> MEDVEIKPRGYQLRLVDHLTKSNGIVYLPTGSGKTFVAILVLKRFSQDFDKPIESGGKRALFMCNTVELARQQAMAVRRCTNFKVGFYVGEQGVDDWTRGMWSDEIKKNQVLVGTAQVFLDMVTQTYVALSSLSVVIIDECHHGTGHHPFREFMRLFTIANQTKLPRVVGLTGVLIKGNEITNVATKLKELEITYRGNIITVSDTKEMENVMLYATKPTEVMVSFPHQEQVLTVTRLISAEIEKFYVSLDLMNIGVQPIRRSKSLQCLRDPSKKSFVKQLFNDFLYQMKEYGIYAASIAIISLIVEFDIKRRQAETLSVKLMHRTALTLCEKIRHLLVQKLQDMTYDDDDDNVNTEEVIMNFSTPKVQRFLMSLKVSFADKDPKDICCLVFVERRYTCKCIYGLLLNYIQSTPELRNVLTPQFMVGRNNISPDFESVLERKWQKSAIQQFRDGNANLMICSSVLEEGIDVQACNHVFILDPVKTFNMYVQSKGRARTTEAKFVLFTADKEREKTIQQIYQYRKAHNDIAEYLKDRVLEKTEPELYEIKGHFQDDIDPFTNENGAVLLPNNALAILHRYCQTIPTDAFGFVIPWFHVLQEDERDRIFGVSAKGKHVISINMPVNCMLRDTIYSDPMDNVKTAKISAAFKACKVLYSLGELNERFVPKTLKERVASIADVHFEHWNKYGDSVTATVNKADKSKDRTYKTECPLEFYDALPRVGEICYAYEIFLEPQFESCEYTEHMYLNLQTPRNYAILLRNKLPRLAEMPLFSNQGKLHVRVANAPLEVIIQNSEQLELLHQFHGMVFRDILKIWHPFFVLDRRSKENSYLVVPLILGAGEQKCFDWELMTNFRRLPQSHGSNVQQREQQPAPRPEDFEGKIVTQWYANYDKPMLVTKVHRELTPLSYMEKNQQDKTYYEFTMSKYGNRIGDVVHKDKFMIEVRDLTEQLTFYVHNRGKFNAKSKAKMKVILIPELCFNFNFPGDLWLKLIFLPSILNRMYFLLHAEALRKRFNTYLNLHLLPFNGTDYMPRPLEIDYSLKRNVDPLGNVIPTEDIEEPKSLLEPMPTKSIEASVANLEITEFENPWQKYMEPVDLSRNLLSTYPVELDYYYHFSVGNVCEMNEMDFEDKEYWAKNQFHMPTGNIYGNRTPAKTNANVPALMPSKPTVRGKVKPLLILQKTVSKEHITPAEQGEFLAAITASSAADVFDMERLEILGDSFLKLSATLYLASKYSDWNEGTLTEVKSKLVSNRNLLFCLIDADIPKTLNTIQFTPRYTWLPPGISLPHNVLALWRENPEFAKIIGPHNLRDLALGDEESLVKGNCSDINYNRFVEGCRANGQSFYAGADFSSEVNFCVGLVTIPNKVIADTLEALLGVIVKNYGLQHAFKMLEYFKICRADIDKPLTQLLNLELGGKKMRANVNTTEIDGFLINHYYLEKNLGYTFKDRRYLLQALTHPSYPTNRITGSYQELEFIGDAILDFLISAYIFENNTKMNPGALTDLRSALVNNTTLACICVRHRLHFFILAENAKLSEIISKFVNFQESQGHRVTNYVRILLEEADVQPTPLDLDDELDMTELPHANKCISQEAEKGVPPKGEFNMSTNVDVPKALGDVLEALIAAVYLDCRDLQRTWEVIFNLFEPELQEFTRKVPINHIRQLVEHKHAKPVFSSPIVEGETVMVSCQFTCMEKTIKVYGFGSNKDQAKLSAAKHALQQLSKCDA;> MDQENFHGSSLPQQLQNLHIQPQQASPNPVQTGFAPRRHYNNLVGLGNGNAVSGSPVKGAPLGQRHVKLKKEKISAQVAQLSQPGQLQLSDVGDPALAGGSGLQGGVGLMGVILPSDEALKFVSETDANGLAMKTPVSILQELLSRRGITPGYELVQIEGAIHEPTFRFRVSFKDKDTPFTAMGAGRSKKEAKHAAARALIDKLIGAQLPESPSSSAGPSVTGLTVAGSGGDGNANATGGGDASDKTVGNPIGWLQEMCMQRRWPPPSYETETEVGLPHERLFTIACSILNYREMGKGKSKKIAKRLAAHRMWMRLQETPIDSGKISDSICGELEGEVSIIQDIDRYEQVSKDFEFIKI

In Drosophila, an RNase III enzyme Dicer-2 (Dcr-2), aided by its cofactor Loquacious-PD (Loqs-PD), has an important role in generating 21 bp siRNA duplexes from long double-stranded RNAs (dsRNAs). ATP hydrolysis by the helicase domain of Dcr-2 is critical to the successful processing of a long dsRNA into consecutive siRNA duplexes. Here six cryo-electron microscopy (cryo-EM) structures of Drosophila Dcr-2–Loqs-PD in apo and in complex with dsRNA substrate in the absence or in the presence of ATP were captured, illuminating the continuous conformational changes of Dcr-2–Loqs-PD after binding to dsRNA and translocating until forming the active dicing state and cleaving the dsRNA substrate into an siRNA duplex in the post-dicing state. Loqs-PD is a cofactor protein that comprises two dsRBDs that are responsible for recruiting siRNA precursor substrates for Dcr-2.

To investigate the dynamic dicing process of Dcr-2, we mixed WT Dcr-2–Loqs-PD with a 50 bp dsRNA substrate, then added ATP and Mg2+ just before generating the cryo-EM samples. From such an enzymatically active sample, we were able to capture a complex structure in the post-dicing state at a relatively lower resolution (4.6 Å). In this structure, a clear breakage of the dsRNA after the dicing near to the catalytic centre was observed and exactly 21 bp away from the PAZ-domain-binding terminus. The cleavage of dsRNA disrupts the binding site for the C-terminal dsRBD in the active dicing state, and probably results in the dsRBD becoming more flexible and losing its density in the averaged EM map of the post-dicing state, which may be also favourable to the release of cleaved siRNA products. Compared with the structure in the active dicing state, the cap–core module with siRNA in the post-dicing state rotated about 20°, which is derived from the partial restoration of the spring helix in the DP-linker, probably accompanied by the release of the tension. The remaining dsRNA duplex bound by the helicase domain also returns to a conformation similar to the early-translocation state, which enables the translocation of Dcr-2–Loqs-PD to enter the next processing cycle. Additional ATP-dependent conformational changes are required to form an active dicing state and precisely cleave the dsRNA into a 21 bp siRNA duplex as confirmed by the structure in the post-dicing state.>[3x]GGSGDEEFSDMLRLFDFNKQAIQRLKAEAQMSIQLINKAVNALIN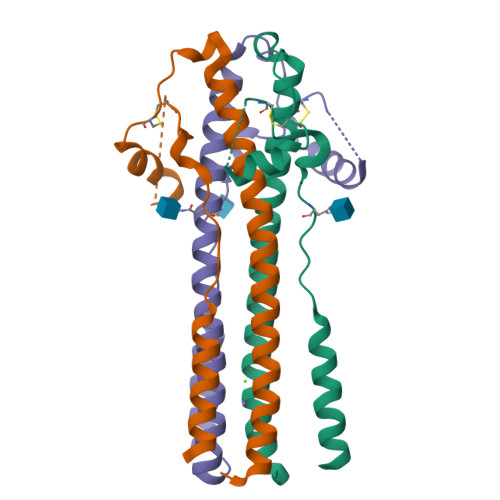DQLIMKNHLRDIMGIPYCNYSKYWYLNHTTTGRTSLPKCWLVSNGSYLNETHFSDDIEQQADNMITEMLQKEY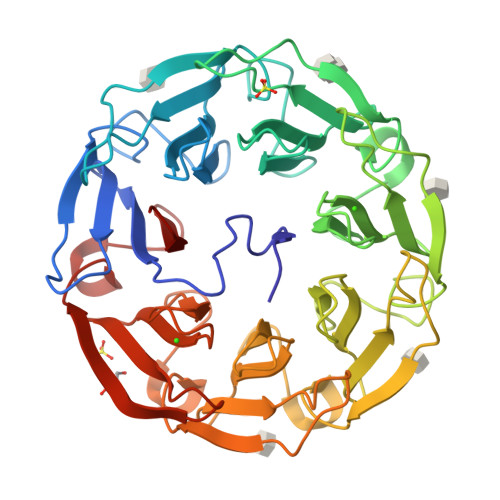> SVVVISQALPVPTRIPGVADLVGFGNGGVYIIRNSLLIQVVKVINNFGYDAGGWRVEKHVRLLADTTGDNQSDVVGFGENGVWISTNNGNNTFVDPPKMVLANFAYAAGGWRVEKHIRFMADLRKTGRADIVGFGDGGIYISRNNGGGQFAPAQLALNNFGYAQGWRLDRHLRFLADVTGDGLLDVVGFGENQVYIARNSGNGTFQPAQAVVNNFCIGAGGWTISAHPRVVADLTGDRKADILGFGVAGVYTSLNNGNGTFGAVNLVLKDFGVNSGWRVEKHVRCVSSLTNKKVGDIIGFGDAGVYVALNNGNGTFGPVKRVIDNFGYNQGWRVDKHPRFVVDLTGDGCADIVGFGENSVWACMNKGDGTFGPIMKLIDDMTVSKGWTLQKTVRYAANLYL> QFLSGQLSIKLWFDKVGHQLIVTILGAKDLPSREDGRPRNPYVKIYFLPDRSDKN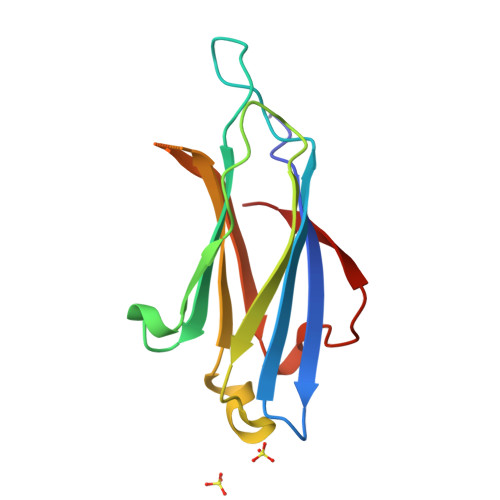KRRTKTVKKTLEPKWNQTFIYSPVHRREFRERMLEITLWDQARVREEESEFLGEILIELETALLDDEPHWYKLQ>[6x]GSFTMASMTGGQQMGRGSMNGDVQSVIRGYLERAQVAKTMSDAGRWNEAGDLLRQLMTDVKSCKISASNRDEHDARNTFLRALEANLKLVQQNVRDEDDLHEAMTRQSGSPEPPADPDVWSKPSPPLPSSSKFGATKKGVGAAGPRPREISKSTSSMSTNPADVKPANPTQGILPQNSAGDSFDASAYDAYIVQAVRGTMATNTENTMSLDDIIGMHDVKQVLHEAVTLPLLVPEFFQGLRSPWKAMV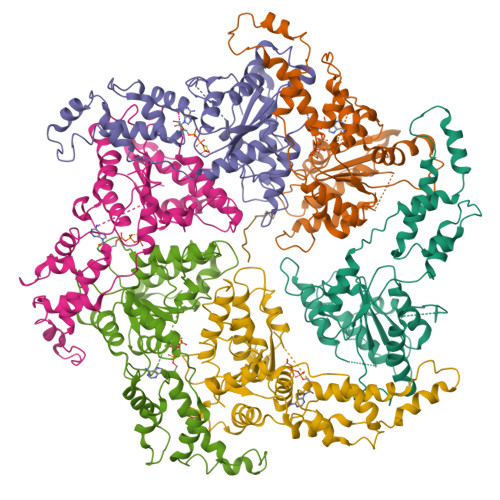LAGPPGTGKTLIARAIASESSSTFFTVSSTDLSSKWRGDSEKIVRLLFELARFYAPSIIFIDQIDTLGGQRGNSGEHEASRRVKSEFLVQMDGSQNKFDSRRVFVLAATNIPWELDEALRRRFEKRIFIPLPDIDARKKLIEKSMEGTPKSDEINYDDLAARTEGFSGADVVSLCRTAAINVLRRYDTKSLRGGELTAAMESLKAELVRNIDFEAALQAVSPSAGPDTMLKCKEWCDSFGAM;> EEEEEEEEEEEE>METDNVELAQSKRKVVLAEQGSFYIGGRTVTGPGKFDPSKPVIPYSNEGATFYINQMYVNFQAPVRPRGLPLVFWHGGGLTGHIWESTPDGRPGFQTLFVQDRHTVYTIDQPGRGRGNIPTFNGPFGQLEEESIVNTVTGNSSKEGAWVRDRLGPAPGQFFENSQFPRGYEDNYFKEMGFSPSISSDEIVDAVVKLVTHIGPCVLVTHAASGVLGMRVATHAKNVRGIVAYEPATSIFPKGKVPEIPPLADKKSQIFPPFEIQESYFKKLAKIPIQFVFGDNIPKNPKSAYWFLDWWRVTRYAHSLSLEAINKLGGQASLLDLPTAGLRGNTHFPFTDRNNVQVASLLSDFLGKHGLDQNESLEHHHHHH[2x]

SulE, an esterase, which detoxifies a variety of sulfonylurea herbicides through de-esterification, provides an attractive approach to remove environmental sulfonylurea herbicides and develop herbicide-tolerant crops. SulE catalyzes the de-esterification of a variety of sulfonylurea herbicides, such as MM, BM, SM, TM, TrM, EM, and CE, to the corresponding herbicidal-inactive parent acid. The structures show that SulE is a dimer with a lid loop in a domain-swapped β-hairpin covering the active site from the opposing monomer. SulE shows a similar catalytic triad consisting of Ser209, His333, and Glu232 at its active site.

To elucidate the catalytic mechanism of SulE, we solved the crystal structures of wild-type SulE in complex with CA, mutant S209A in complex with MM, and mutant S209A/H333A in complex with MM, SM, TM, TrM, EM, BM, and CE in the range of 1.29–1.63 Å. In the S209A-MM complex structure, clear electron density was observed for the benzene ring of MM, but the electron density for the sulfonylurea bridge and the heterocyclic ring was unclear, probably due to the considerable mobility of the flexible sulfonylurea bridge. By contrast, the sulfonylurea bridge and the heterocyclic ring of MM was clearly observed and well localized to the active site of S209A/H333A, indicating that MM binds more stably in S209A/H333A than in S209A. In the S209A-MM complex structure, the benzene ring is also surrounded by some hydrophobic residues Ile43, Ala234, Phe257, Phe293, Trp296, and Trp297. The sulfonylurea bridge also forms hydrogen bonds with two hydrophilic residues Tyr45 and Arg150, and the heterocyclic ring also forms a π-π interaction with Phe257. However, it was found that the SulE S209A and P44R/S209A mutants still retained weak activity in this study. The distance between His333 and the substrate is too long to have a direct reaction; therefore, the reason why SulE S209A and P44R/S209A mutants still retain de-esterification activity may be that a water molecule got into the active site and was directly deprotonated by His333 when Ser209 is mutated to alanine, and then as a nucleophile to attack the ester bond of the substrate.> MAIIAGKAGYGLIIALFSLSLSGCGLTQR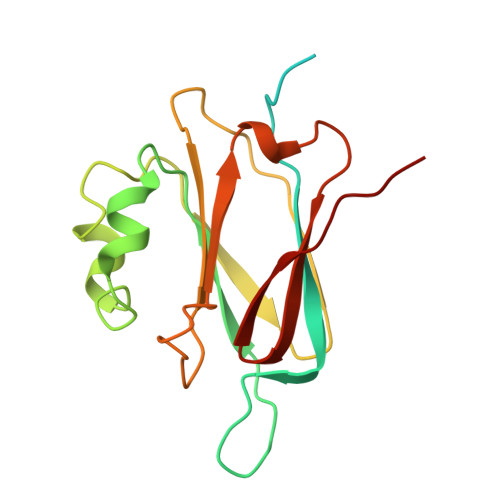VADGTVSATKSLFYRQIKTLHLDIRAREAINTSAAGIPLSVVVRIYQLKDNRSFDSADYQALFTGDNEILAGDIIAQKDVWLQPGGSVAVDMPLDDAAKFTGVAAMFLEPDQKKNTWRVVLGRDELEPDTPRLIEVSGNTLTLLPVKDK> PGGTR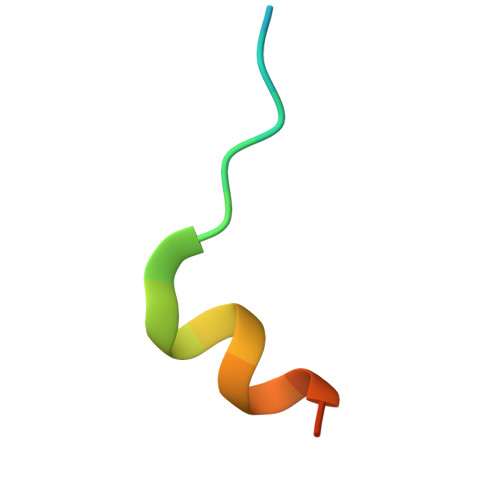IIYDRKFLMECRNSP>[2x]QDSTSDLIPAPPLSSVPLQQNFQDNQFQGKWYVVGLAG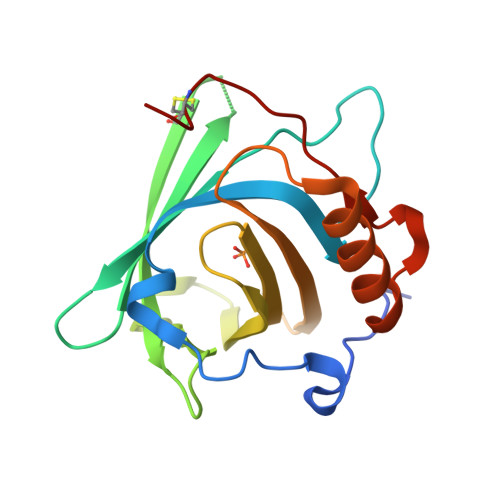NAILREDEDPQKMYATIYELKEDKSYNVTSVLFRDDGCDYWIRTFVPGCQPGEFTLGNIQSYPGLTSYLVRVVSTNYNQFAMVFFKKVSQNQEYFKITLYGRTKELTSELQENFIRFSKSLGLPENNIVFPVPIDQCIDG> MKDKVYKRPVSILVVIYAQDTKRVLMLQRRDDPDFWQSVTGSVEEGETAPQAAMREVKEEVTIDVVAEQ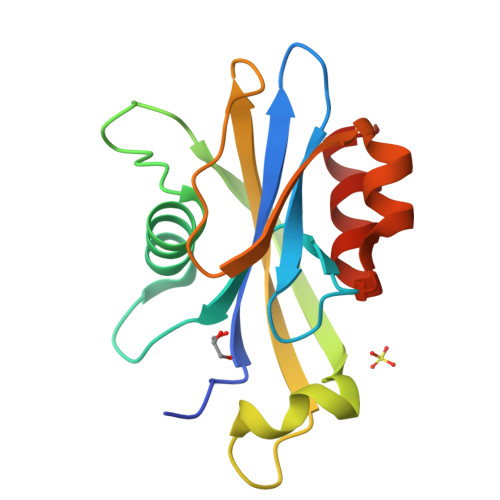LTLIDCQRTVEFEIFSHLRHRYAPGVTRNTESWFCLALPHERQIVFTEHLAYKWLDAPAAAALTKSWSNRQAIEQFVINAA>[2x]GSHMTEGTIKTSKYEIIAIFREELRKRTEIEI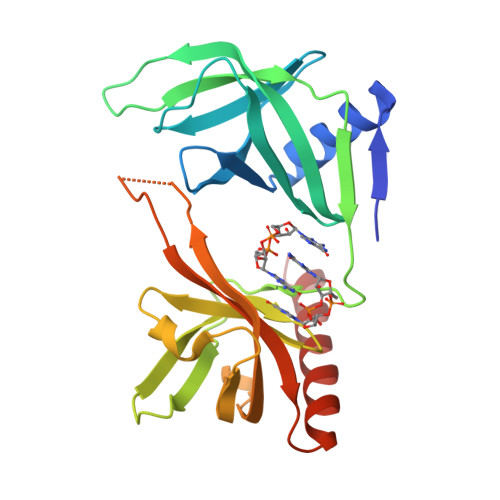FFNNTSIITQLTRVDFAEFHIQTHRKIPSGHKIRFLLHSDSGKIEFNAALTKHDNSGVDKGIRYAFSLPECLQVVQRRRDPRFRLRAEHDFYCRGRHKNGENYLFDIKDISDGGCALMTKTPNLKFLSHDALLKNAVLMLAEYGEITIDLVVKNVIVITLDNANEESESYYQISCQFKFRHLDDQRRIEKILLDLILEAKRKK pentan-2-one 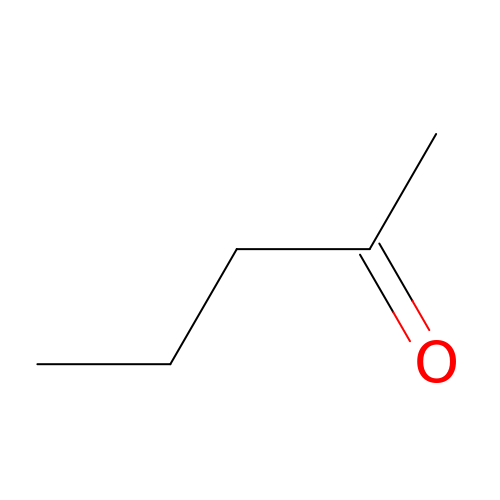| C5 H10 O | XNLICIUVMPYHGG-UHFFFAOYSA-N>[2x]GPLPAHDASKVRASGPGLNASGIPASLPVEFTIDARDAGEGLLTVQILDPEGKPKKANIRDNGDGTYTVSYLPDMSGRYTITIKYGGDEIPYLPFRIHA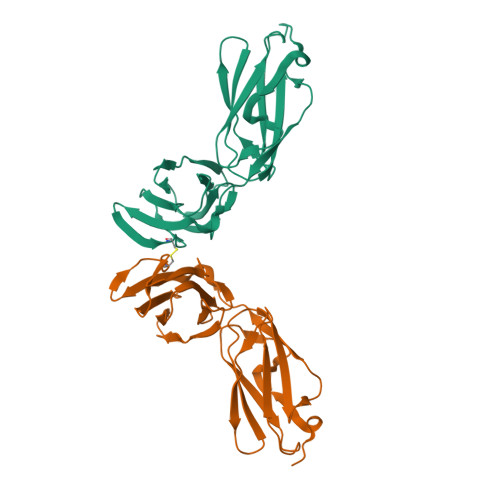LPTGDASKCLVTVSIGGHGLGACLGPRIQIGQETVITVDAKAAGEGKVTCTVSTPDGAELDVDVVENHDGTFDIYYTAPEPGKYVITIRFGGEHIPNSPFHVLATE>MAENDFGIAIIGMAGRFPQADTVQAFWENLLASRECISFYSDEELLAMGISPEFVQHPDYVKAKGEVADIDKFDAAFFGIAPREAELMDPQHRVLLETAWAAFEDAGYVAADYPGDVGIFAGKSMDSYLMLNLMPHFKRVFSSGSLQAAIGNDKDSITTTIAYHLNLRGPAITVQTSSSTSLVAVCVACQSLLTWQCDMAIAGGVTLGPPAKTGYLSQEGGITAADGHCRAFSDNSSGFVPGTGAGLVVLKRVDEALRDGDNIYAVIKGFAVNNDGSEKISYTAPSVDAQARAIAQAQRLAGLTPQDITYVEAHGTGTRLGDPVEFSALSQAFAGASQKQYCALGSVKTNIGHLDTAAGVAGLIKTALAVQQGIIPATLHFERPNAQIDLTNSPFYINTTCQPWQPESGIRRAGVTSLGMGGTNAHVVLEQAPAVDLQARAPVPAYSILPFSAKTDSALSSGLARFADFLQHESLPDRRDLAWTLSQGRKAFAHRAALVTRDLHAAGTLLQQAATAPFARGVAQTQLGLGLLFSGQGSQYQRMGHQLYQVWPA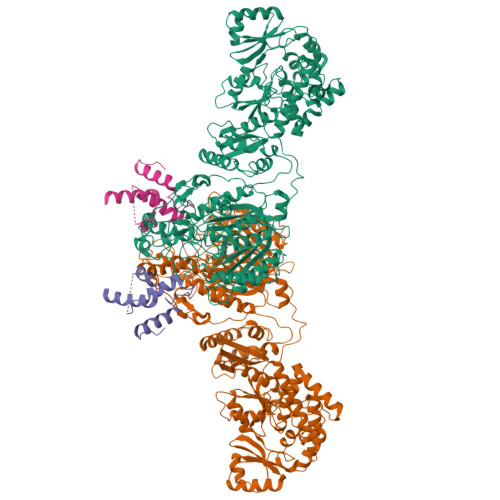YADAFDRCATLLEREYQLDIRHELFRAEVSLAQGERLAQTCLTQPLLFSVEYALAQLWLSWGITPTVMIGHSLGEWVAATLAGVFSLEDALRLVARRAELMHQAPSGAMLMVALPEAQIRALITAPLAIAAVNAPDYSVIAGPTSEILAVSQRLTEQNIINKRLHTSHAFHSSMMQDAAQALRQAFENVRLNPPTLTIISTVTGAHVSADTLTTPDYWIEQMLMPVQFSAALQEAQATFDVDFLEIGPGATLTQLTNGHALGDRLAFSSLPAGARSSDEHKHILDTVAALWVRGHNIDLSAFAGEQPRRVSLPTYAFDKIRYWVDSPEEQRSAVTPVADAGSKLSSGLEVLFQGPSSGHHHHHHHHHH[2x];>[2x]VIPSEPSVRRQPRPAFSVPYAAPESKTQRGLVAICEALLGIDGLGIDDNFFEAGGHSLMLGMLLAQVQERFAVTLSFFDVMEDASVRALAQLVEQEQQDDGGSALAVLVNDMINEKLSSGLEVLFQGPSSGHHHHHHHHHH>[2x]DEDDWSKPLPPSERLEQELFSGGNTGINFEKYDDIPVEATGNNCPPHIESFSDVEMGEIIMGNIELTRYTRPTPVQKHAIPIIKEKRDLMACAQTGSGKTAAFLLPILSQIYSDGPGEALRAMKENGRYGRRKQYPISLVLAPTRELAVQIYEEARKFSYRSRVRPCVVYGGADIGQQIRDLER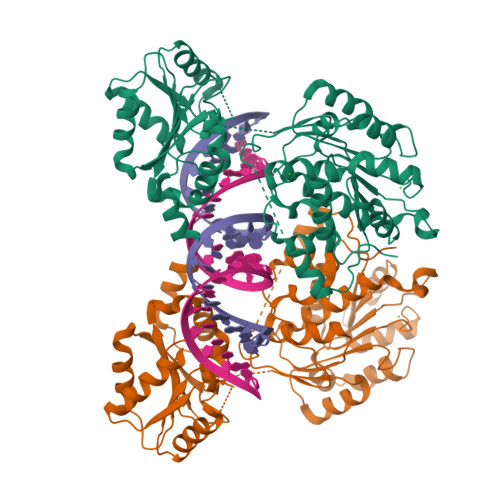GCHLLVATPGRLVDMMERGKIGLDFCKYLVLDEADRMLDMGFEPQIRRIVEQDTMPPKGVRHTMMFSATFPKEIQMLARDFLDEYIFLAVGRVGSTSENITQKVVWVEESDKRSFLLDLLNATGKDSLTLVFVETKKGADSLEDFLYHEGYACTSIHGDRSQRDREEALHQFRSGKSPILVATAVAARGLDISNVKHVINFDLPSDIEEYVHRIGRTGRVGNLGLATSFFNERNINITKDLLDLLVEAKQEVPSWLENMAYEHHYKGSSRGRSKSSRFSGGFGARDYRQSSG>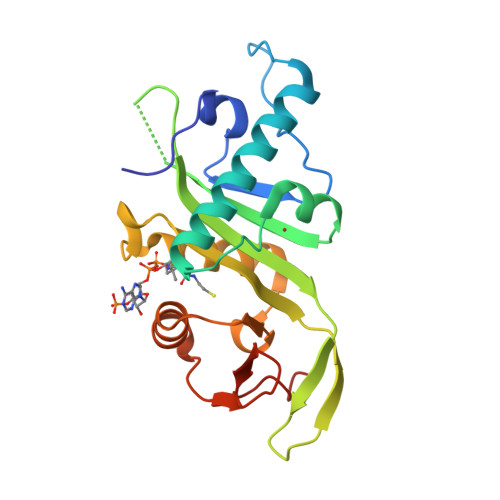 GPGSMEFPFDVDALFPERITVLDQHLRPPARRPGTTTPARVDLQQQIMTIIDELGKASAKAQNLSAPITSASRMQSNRHVVYILKDSSARPAGKGAIIGFIKVGYKKLFVLDDREAHNEVEPLCILDFYIHESVQRHGHGRELFQYMLQKERVEPHQLAIDRPSQKLLKFLNKHYNLETTVPQVNNFVIFEGFFAHQHEFG>[12x]MNYATVNDLCARYTRTRLDILTRPKTADGQPDDAVAEQALADASAFIDGYLAARFVLPLTVVPSLLKRQCCVVAWFYLNESQPTEQITATYRDTVRWLEQVRDGKTDPGVESRTAASPEGEDLVQVQSDPPVFSRKQKGFI;>MGRILDISG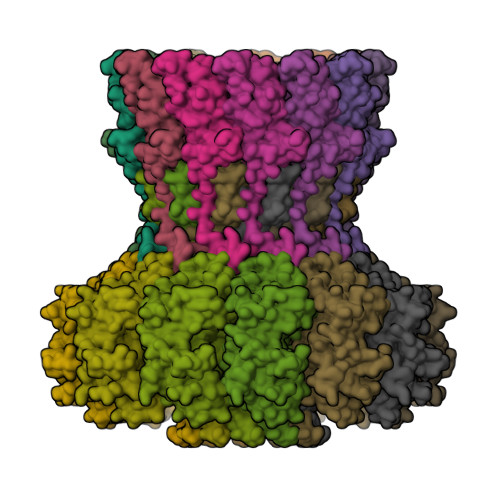QPFDFDDEMQSRSDELAMVMKRTQEHPSSGVTPNRAAQMLRDAERGDLTAQADLAFDMEEKDTHLFSELSKRRLAIQALEWRIAPARDASAQEKKDADMLNEYLHDAAWFEDALFDAGDAILKGYSMQEIEWGWLGKMRVPVALHHRDPALFCANPDNLNELRLRDASYHGLELQPFGWFMHRAKSRTGYVGTNGLVRTLIWPFIFKNYSVRDFAEFLEIYGLPMRVGKYPTGSTNREKATLMQAVMDIGRRAGGIIPMGMTLDFQSAADGQSDPFMAMIGWAEKAISKAILGGTLTTEAGDKGARSLGEVHDEVRREIRNADVGQLARSINRDLIYPLLALNSDSTIDINRLPGIVFDTSEAGDITALSDAIPKLAAGMRIPVSWIQEKLHIPQPVGDEAVFTIQPVVPDNGSQKEAALSAEDIPQEDDIDRMGVSPEDWQRSVDPLLKPVIFSVLKDGPEAAMNKAASLYPQMDDAELIDMLTRAIFVADIWGRLDAAADH[12x]>MSGDNGVYSGSAAYNTATAPKVPVSRATFFQNTKSKDFDFKFADGADAIANVLQQMEHGVAQHQLGDMNVRTDGLATVSAVLNGRKRKIANQYMMHFDLFGRAARSTVRMESRIQSFGEGKDVDNFMAKFHNQLSGVYERRSEGVANFGRILATDTDLGGTSGLSVVFNGLLRGLHHVSTVPTPNVANLPIRNNRDGAGAVVGRGDMPGREFMDSSRILPPRSSRWYGAPGQPIVPPAPNNPPAHVAPMETVMAGLQKTVMNELNRVIVSIADVPKLPAHRIRNLIAVLAAVSKPNLGFDANRLEDHSCFTKGWLGF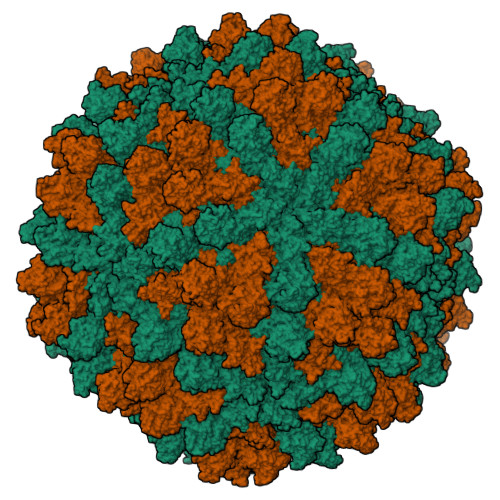NDILLFPLTVDLFDRVVANEAGVNDAGFIVPNAAPPQFLQNTNQQVIDFRGVGVGQAGDIPALRLAQSWSDAIGFLLDTIGGEAQLAMGLNDMVAQCFHMHGAQTTMLSTPIISRADFGVYHNVVTNMYRRLAYMYTRLIRTNAAAGGGAMLDRQHYQWPTHAKVGFHDDTAVNAAAAAARIHDGLRQPLLDEAFGAGVVQPGNMDLVGAGIDFTRDLTSSLGKAYPEHRPIGADDNKRDLGDFTAGTVDAAASGYEWDNYVYRLFGNMSAMRSKAEFDRLLATFPSSTLSELFIWMGNVGFADTWEERWGYDAAPLCSIPIPAGHDRSMLRNWSWVNVHNVHSVTGTSENVVLAGYVGLSRTHDYIMDTRSTPATSQGRRLAAMFYYTNADKMLSLTFGLAGQLRAAADTTVAKFQICPHTIARAQGYIMTDNDPLSDELKGTDFVTEQFSLAGLTNLYLGYFDGLATRLGIYDLRYTYSEYAECRVELHGIQRNFLTDRLDAFVSYKCLHPIMFEYYMCGANISGGILNGDKAYEQVEMGNIRAYDAMFDTSAARDFNFVGVRGASQQIAAVGGFHIQYKMEVEIQRPGDGTEASRFNVYERYLNNYLRMSDCAPTSVLNAVSPLFWMAGTTRVVLCEAANGYKPMAYDISQTSFWNRENGLWAFTWGESEKTHRPNAIPHGTRRLGNSEVLMNSRFSKILDKKGITKLETRVGGRKRGDNNDDFVAADTRMFIIQDVAGGEHAAYSSLRDPGFALVRAAHTWDTFVQNPRMLLLERGYGNTGFTDTYSAAGIRRTNGHISLRLSALTDDFEFTMHPLARAEYKETSRVSLTSMIYVGTAGKDLSLPTGTVEDIIGAVDGMRRVVRTIGGQTIKTAPVVPPTEQRDMVQEERVGTPVKNAGNANPAADSDNATEGVVEPKN[2x]(2S)-hexane-1,2,6-triol | C6 H14 O3 | 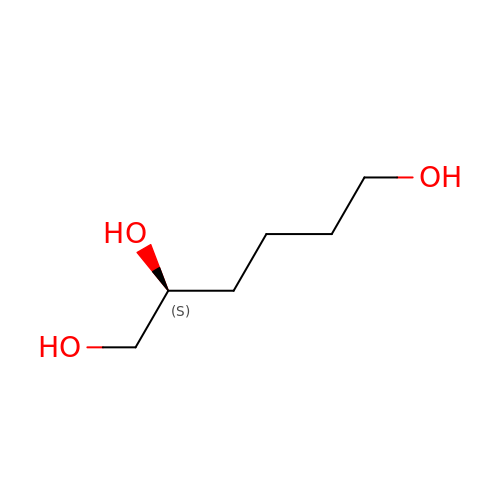ZWVMLYRJXORSEP-LURJTMIESA-N Among families of proteins involved in signal transduction, phospholipase C (PLC) enzymes that generate second messengers from phosphatidylinositol 4,5-bisphosphate (PIP2) incorporate a number of different protein modules. PLCγ enzymes (PLCγ1 and PLCγ2), for example, contain eight domains, four of which are unique to this PLC family (Bunney and Katan, 2011; Suh et al., 2008). The PLCγ ‘specific array’ of domains (γSA), comprising a “split” PH (spPH) domain flanking two tandem SH2 domains and an SH3 domain, is inserted between the two halves (X and Y) of the TIM-barrel catalytic domain (Bunney and Katan, 2011). We demonstrate that among four domains present in the γSA, the cSH2 domain and its C-terminal linker provide a focus for most interdomain interactions both within the γSA and between the γSA and the PLC-core.

To analyze the structural and functional implications of Y783 phosphorylation and the potential for intramolecular binding to cSH2, we obtained the crystal structure of a construct incorporating nSH2-cSH2Y771F,Y775F (545–790) following phosphorylation on Y783. The structure of the tandem protein revealed an intramolecular interaction between the cSH2 canonical pY-peptide binding site and residues 781GFpYVEANPM790. Residues 774 to 780 are not visible in the electron density map suggesting that this part of the linker remains disordered. The structure shows that the cSH2 domain makes an essentially canonical binding interaction with the extended linker in which the pY783 side chain makes multiple interactions with three arginine (R675, 694, and 696) side chains in the conserved pY-binding pocket. The side chains of residues pY+1 (V784) and pY+3 (A786) are directed into shallower, hydrophobic pockets (formed by cSH2 residues F706, L726, L746, and Y747). The side chains of V784, A786, and P788 all make van der Waals contacts with the cSH2 domain, burying ∼620 Å2 of solvent accessible surface. Although the structure of the cSH2 domain is not affected upon pY783 binding, a further, more detailed comparison of the crystal structure of the phosphorylated nSH2-cSH2 protein with the nonphospho (apo) construct in the same crystal form shows general similarity with some subtle differences in angle and distance between the domains (not shown). However, the second binding phase is highly suppressed due to occupancy in cis of the canonical pY-binding site on the cSH2 by the pY783-linker region. The cSH2, in contrast, makes contacts with the PLC-core and recognizes an intramolecular pY motif rather than a receptor site. It also seems that a relatively small change in the tandem cSH2-nSH2—induced upon pY783 binding to cSH2—is allosterically relayed to the nSH2 domain reducing the affinity for FGFR1 but with no corresponding allosteric effect on PLC activity.

>HSNEKWFHGKLGAGRDGRHIAERLLTEYCIETGAPDGSFLVRESETFVGDYTLSFWRNGKVQHCRIHSRQDAGTPKFFLTDNLVFDSLYDLITHYQQVPLRCNEFEMRLSEPVPQTNAHESKEWYHASLTRAQAEHMLMRVPRDGAFLVRKRNEPNSYAISFRAEGKIKHCRVQQEGQTVMLGNSEFDSLVDLISYYEKHPLYRKMKLRYPINEEALEKIGTAEPDFGALFEGRNPGFYVEANPMP[4x]>GGACCTTGGTCC[2x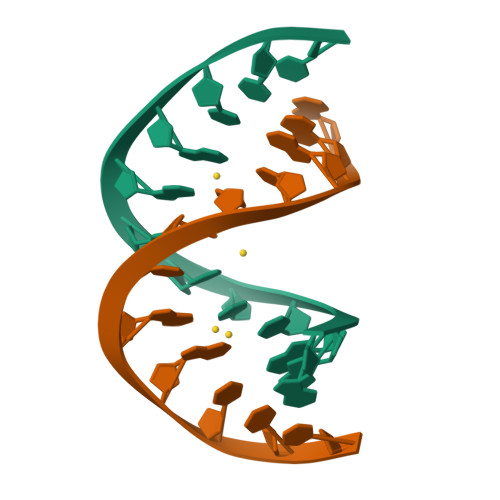]>[6x]SHMPPRYTDQGGEEEEDYESEEQLQHRILTAALEFVPAHGWTAEAIAEGAQSLGLSSAAASMFGKDGSELILHFVTQCNTRLTRVLEEEQKLVQLGQAEK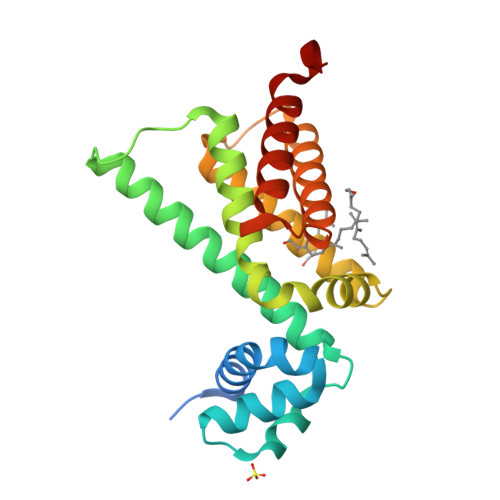RKTDQFLRDAVETRLRMLIPYIEHWPRALSILMLPHNIPSSLSLLTSMVDDMWHYAGDQSTDFNWYTRRAMLAAIYNTTELVMMQDSSPDFEDTWRFLENRVNDAMNMGHTA> MTEGAKKAPVIWVQGQGCTGCSVSLLNAVHPRIKEILLDVISLEFHPTVMASEGEMALAHMYEIAEKFNGNFFLLVEGAIPTAKEGRYCIVGETLDAKGHHHEVTMMELIRDLAPKSLATVAVGTCSAYGGIPAAEGNVTGSKSVRDFFADEKIEKLLVNVPGCPPHPDWMVG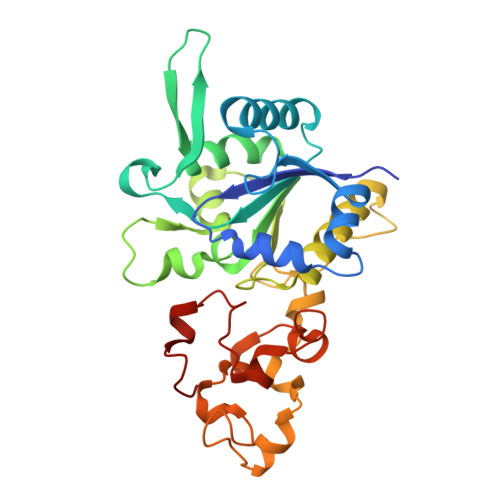TLVAAWSHVLNPTEHPLPELDDDGRPLLFFGDNIHENCPYLDKYDNSEFAETFTKPGCKAELGCKGPSTYADCAKRRWNNGINWCVENAVCIGCVEPDFPDGKSPFYVAE>QSVKESEGGLFKPTDTLTLTCTASGFSLNGYGVIWVRQAPGKGLEWIGSAGAYGRIYYPNWARSRATITRNTNLNTVSLKMTSLTAADTATYFCARRTNVSTSVGFDSWGPGTLVTVSSSSGQPKAPSVFPLAPCCGDTPSSTVTLGCLVKGYLPEPVTVTWNSGTLTNGVRTFPSVRQSSGLYSLSSVVSVTSSSQPVTCNVAHPATNTKVDKTVAPSTCSHHHHHH[6x];>[6x]DMTQTPSSKSVPVGDTVTINCQASESVYSNNRLSWFQQKPGQPP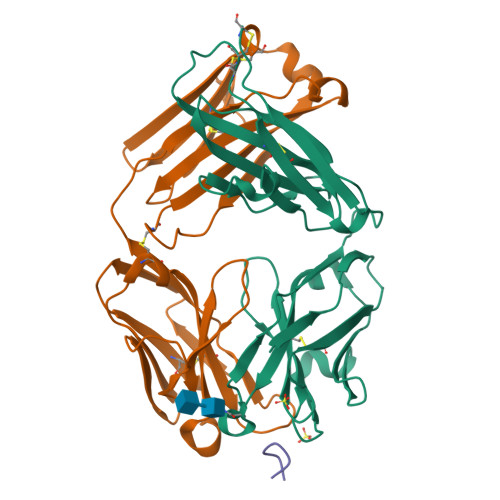KLLIYLVSTLASGVPSRFKGSGSGTQFTLTISDVVCDDAATYYCVGYKSSTTDGLAFGGGTEVVVKGDPVAPTVLIFPPAADQVATGTVTIVCVANKYFPDVTVTWEVDGTTQTTGIENSKTPQNSADCTYNLSSTLTLTSTQYNSHKEYTCKVTQGTTSVVQSFNRGDC;>[6x]RNIIXGSDS Adenosine triphosphate (ATP), the fuel of life, is produced in inner membranes of the mitochondria of eukaryotic cells by an embedded molecular machine with a rotary action, called ATP synthase. Mitochondrial ATP synthases occupy the inner membranes of the organelle and form dimers via specific interactions in their membrane domains. Each monomeric unit in the dimeric bovine enzyme described here is an assembly of 28 polypeptide chains of 17 different kinds, organized into a spherical catalytic globular domain that extends from the inner mitochondrial membrane (IMM) into the mitochondrial matrix, attached to an intrinsic membrane domain by a central stalk and a peripheral stalk (PS). This membrane-bound enzyme is a machine that transmits by a rotary action the potential energy of the transmembrane proton motive force, generated by respiration, into the catalytic sites in the extrinsic domain.

The membrane-bound rotor consists of a ring of eight identical c-subunits in close association with a single static a (or ATP-6) subunit, attached to the asymmetrical central stalk (subunits γ, δ, and ε) which extends from the membrane domain and penetrates into the extrinsic globular catalytic domain along its central axis. Focused local refinement of the rotor (c8-ring plus subunits γ, δ, and ε), the stator (subunits OSCP, b, d, and F6 and associated supernumerary subunits e, f, and g) and the membrane domain (subunits a, A6L, b, d, e, f, g, j, k, and the c8-ring) improved the quality of the maps and the resolutions in these regions to 3.5 to 3.7, 4.2 to 6.0, and 3.6 Å. As it rotates, the asymmetrical central stalk brings about structural changes in the three catalytic sites, found mainly in each of the three β-subunits, which alternate with three noncatalytic α-subunits in the spherical extrinsic domain. The inhibition of ATP hydrolysis in the isolated catalytic F1-domain arrests the rotary cycle at the catalytic dwell, and in structures of the inhibited bovine F1-IF1 complex, the rotary cycle has been arrested at 27° to 32° after the pause in the rotary cycle preceding the release of phosphate. In the current structure, the postphosphate release angles are 28.8°, 26.2°, and 25.5° in states 1 to 3, respectively. Therefore, the rotational angle in the F1-domain is not influenced significantly by interactions with the additional components of the intact enzyme that are absent from the isolated F1-domain. The central cavity of the c8-ring contains a poorly defined, noisy density observed also in the porcine and yeast c-rings (S13 A–E). Here, the upper half of this density has been attributed to a mobile lipid (including possibly coenzyme Q10), and the lower half has been ascribed to another mobile lipid and the C-terminal region of the e-subunit, which extends toward the central cavity on the inter-membrane space (IMS) side of the membrane and could just penetrate into the cavity.

> ATLKDITRRLKSIKNIQKITKSMKMVAAAKYARAERELKPARVYGVGSLALYEKADIKTPEDKKKHLIIGVSSDRGLCGAIHSSVAKQMKSEAANLAAAGKEVKIIGVGDKIRSILHRTHSDQFLVTFKEVGRRPPTFGDASVIALELLNSGYEFDEGSIIFNRFRSVISYKTEEKPIFSLDTISSAESMSIYDDIDADVLRNYQEYSLANIIYYSLKESTTSEQSARMTAMDNASKNASEMIDKLTLTFNRTRQAVITKELIEIISGAAALD;> AEAAAAQAPAAGPGQMSFTFASPTQVFFNSANVRQVDVPTQTGAFGILAAHVPTLQVLRPGLVVVHAEDGTTSKYFVSSGSVTVNADSSVQLLAEEAVTLDMLDLGAAKANLEKAQSELLGAADEATRAEIQIRIEANEALVKALE;> VAYWRQAGLSYIRYSQICAKAVRDALKTEFKANAMKTSGSTIKIVKVKKE;>[8x]DIDTAAKFIGAGAATVGVAGSGAGIGTVFGSLIIGYARNPSLKQQLFSYAILGFALSEAMGLFCLMVAFLILFAM>APQQINDIVHRTITPL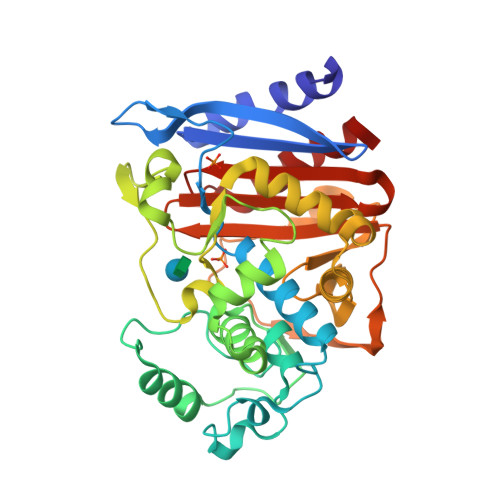IEQQKIPGMAVAVIYQGKPYYFTWGYADIAKKQPVTQQTLFELGGVSKTFTGVLGGDAIARGEIKLSDPTTKYWPELTAKQWNGITLLHLATYTAGGLPLQVPDEVKSSSDLLRFYQNWQPAWAPGTQRLYANSSIGLFGALAVKPSGLSFEQAMQTRVFQPLKLNHTWINVPPAEEKNYAWGYREGKAVHVSPGALDAEAYGVKSTIEDMARWVQSNLKPLDINEKTLQQGIQLAQSRYWQTGDMYQGLGWEMLDWPVNPDSIINGSDNKIALAARPVKAITPPTPAVRASWVHKTGATGGFGSYVAFIPEKELGIVMLANKNYPNPARVDAAWQILNALQ[2x]>MSEIVKFNPVMASGFGAYIDHRDFLEAKTETIKNLLMRQGFVVVKNLDIDSDTFRDIYSAYGTIVEYADEKIGVGFGYRDTLKLEGEKGKIVTGRGQLPFHADGGLLLSQVDQVFLYAAEIKNVKFRGATTVCDHALACQEMPAHLLRVLEEETFEVRVLERGYYVDVSPDGWFKVPVFTDL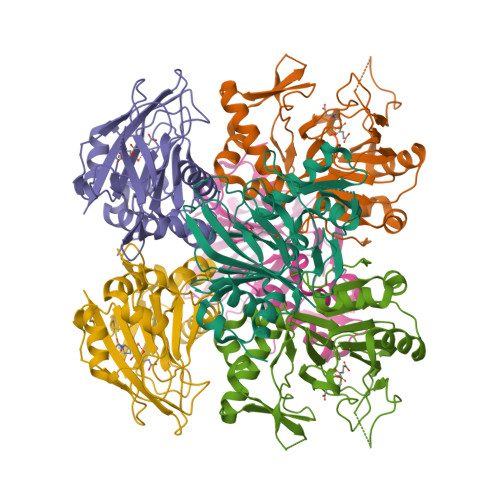GWVRKMLIYFPFDEGQPASWEPRIVGFTDHETQAFFQELGAFLKQPRYYYKHFWEDGDLLIMDNRRVIHEREEFNDDDIVRRLYRGQTADI[3x]>MGSDKIHHHHHHMDVFSDRVLLTEESPIRKLVPFAEMAKKRGVRIHHLNIGQPDLKTPEVFFERIYENKPEVVYYSHSAGIWELREAFASYYKRRQRVDVKPENVLVTNGGSEAILFSFAVIANPGDEILVLEPFYANYNAFAKIAGVKLIPVTRRMEEGFAIPQNLESFINERTKGIVLSNPCNPTGVVYGKDE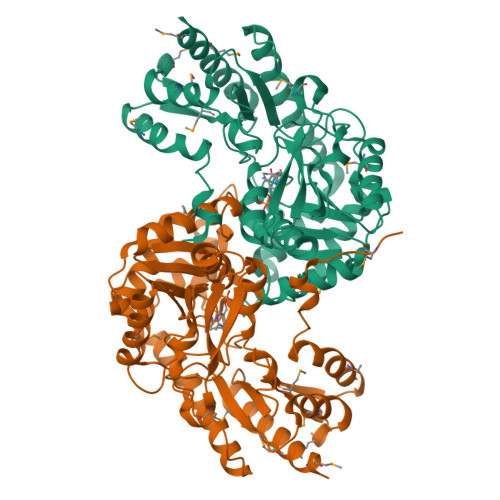MRYLVEIAERHGLFLIVDEVYSEIVFRGEFASALSIESDKVVVIDSVSKKFSACGARVGCLITRNEELISHAMKLAQGRLAPPLLEQIGSVGLLNLDDSFFDFVRETYRERVETVLKKLEEHGLKRFTKPSGAFYITAELPVEDAEEFARWMLTDFNMDGETTMVAPLRGFYLTPGLGKKEIRIACVLEKDLLSRAIDVLMEGLKMFCSSRISC[6x]ethyl 4-{3-[(2,4-diamino-5-methylpyrido[2,3-d]pyrimidin-6-yl)methyl]-4-methoxyphenoxy}butanoate | C22 H27 N5 O4 | 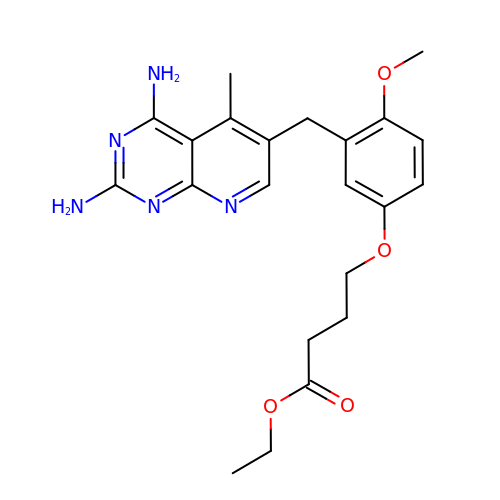OJXNTDHQQMJPKJ-UHFFFAOYSA-N>[2x]QEGTLERSDWRKFFSEFQAKGTIVVADERQADRAMLVFDPVRSKKRYSPASTFKIPHTLFALDAGAVRDEFQIFRWDGVNRGFAGHNQDQDLRSAMRNSTVWVYELFAKEIGDDKARRYLKKIDYGNADPSTSNGDYWIEGSLAISAQEQIAFLRKLYRNELPFRVEHQRLVKDLMIVEAGRNWILRAKTGWEGRMGWWVGWVEWPTGSVFF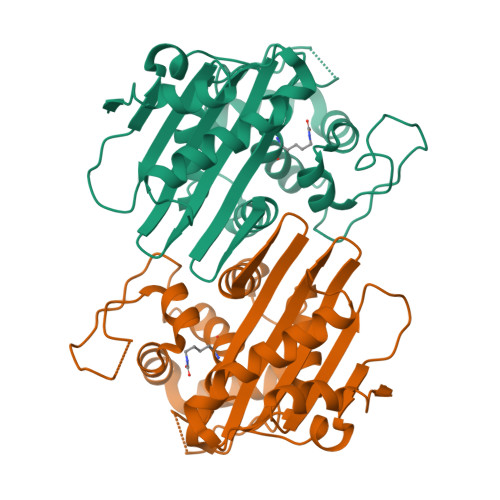ALNIDTPNRMDDLFKREAIVRAILRSIEALPPNPAVNSDAAR> SGSMAAGERWWRFRVDYHAGPMDDLILDGVRPAFAAFAAQAPMAYFLRHWRRGPHLRIYVSTTREALEAVVRPAIEHVVGGYLRARPSPGMADPSAFLPLHERLAELEGEDGPLMPWSPDNTIHAEGERPEPLTVRDVLLADFYADTTPSVYHALERVRSGASLPTIAFDLVVATAHALSTGGLPVARTSLRSHAEAYLARRSDGVRLRELWRDHYARNREAFTERLIAVASSAESAENGAHLPHVREWVRRLRPIRERARALLESGELTLEYASPAEGARDLPSLAEVSAFHRELESRPEWARLRDSPAFGAYRLVINCTYLHLTRLGLTPH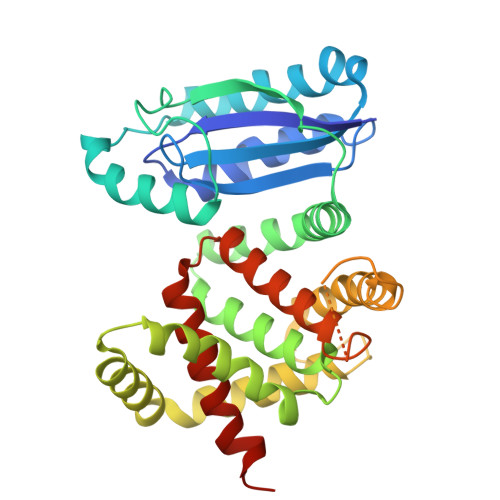QRFLVCHLAADAAADVYGIAAHEEVATR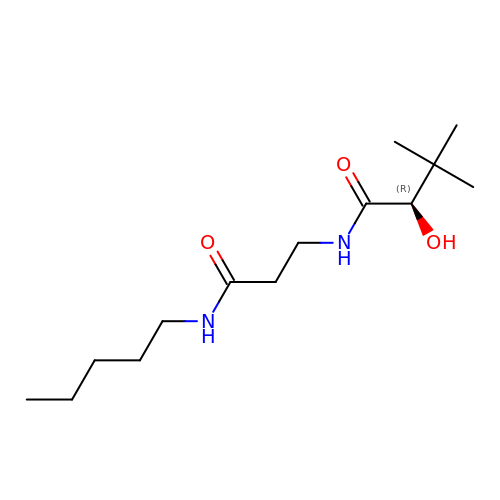(2R)-2-hydroxy-3,3-dimethyl-N-[3-oxo-3-(pentylamino)propyl]butanamide | C14 H28 N2 O3 | ZNKPIBQTIYRSDI-LBPRGKRZSA-N> MGNVLVVIEQRENVIQTVSLELLGKATEIAKDYDTKVSALLLGSKVEGLIDTLAHYGADEVIVVDDEALAVYTTEPYTKAAYEAIKAADPIVVLFGATSIGRDLAPRVSARIHTGLTADCTGLAVAEDTKLLLMTRPAFGGNIMATIVCKDFRPQMSTVRPGVMKKNEPD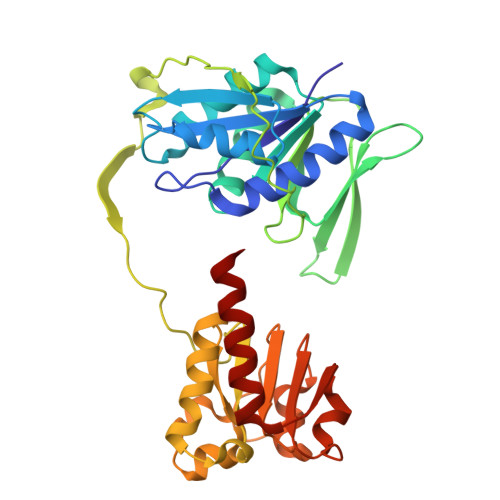ETKEAVINRFKVEFNDADKLVQVVQVIKEAKKQVKIEDAKILVSAGRGMGGKENLDILYELAEIIGGEVSGSRATIDAGWLDKARQVGQTGKTVRPDLYIACGISGAIQHIAGMEDAEFIVAINKNPEAPIFKYADVGIVGDVHKVLPELISQLSVAKEKG>[4x]MSTVTTINLEDIKEICHTTIRLGGKPESGEAAELPIFLGS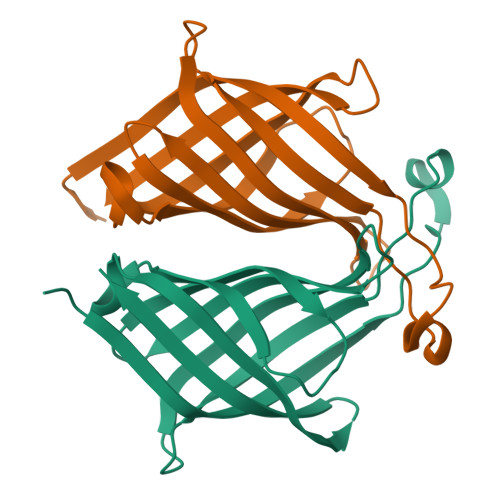SVEFEDELYDADGTQIGTAKGTSVIFAEADGTVMQIVSAFDDYTDGGRVTWSGAYTMFPTDEPKSVPAQGVSGRYRGLSGTRTFQLLERPDPGTSLIRSSLVLNG>[2x]MEAEKKLFLKALKEKFEEDPKEKYTKFYTFGGWQQSARKREFVEANEKIVAEKRGGIPMYNPDIGVPLGQRKLMPYKLSGTDYIVEGDDLHFMNNAAIQQMWDDIRRTVIVGMDTGHAVLEKRLGVEVTPETINEYMATINHSLPGGAVVQEHMVEVHPSLAWDCYAKIFTGDDELADELDKKYLIDINKLFPEEQAEQLKAAIGKKTYQVSRVPTLVGRVCDGGTIARWSAMQIGMSFITAYKLCAGEAAIADFSYAAKHADVVGVGTALPARRSRGANEPGGIPFGVLCDIVQTTRISDDPVEQSLEVVAVGAMLYDQVWLGSYMSGGVGFTQYATAAYTDDILDDFAYYGYEYVEKKYGINSTKPTMDVVEDIATEVTLYSLEQYDEFPTLLEDHFGGSQRAAVAAAASGISVCMATGNSNAGVNGWYLSQIMHKEYHSRLGFYGYDLQDQCGASNSLSIRNDEASPLELRGPNYPNYAMNVGHQGEYAGITQAAHSARKDAFAMNPLIKIAFADPSLVFDFARPRKECARGALREFEAAGERDVILPAK;>[2x]MVKYEDKISLYDAKGNLVEDGVPLEAISPL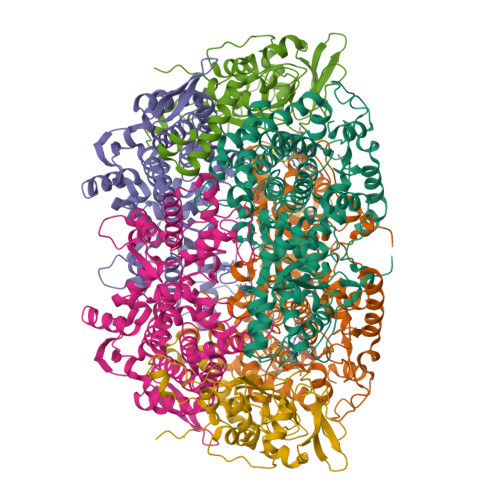YNPTIKAMVKNIKRTVAVNLAGIENSLKTGAIGGKGCKVPGRTLDLPIVENAEAIMDEVEKILRITPDDDTQLRAINDGKQLVVQVPSKRLEVAAEYSVSMLNTAMALKEAIIKTFDVDLFDGSTIHAAIVGRYPQVMDYMGGNIASLLGAPSNMEGLGYALRNIMVNHYVATTKKNLMNAVAFASIMEQTAMFEMGDAIGSFERMHLLGLAYQGLNSDNLVIDLVKANSKGTVGTVVASVVERALEDKVIVEDKSLESGFTMYKPADVAKWNAYAAAGLVAAVIVNCGAARAAQNVASTILYYNDILEYETGLPGTDFGRAEGTAVGFSFFSHSIYGGGGPGIFTGNHVVTRHSKGFAIPPVCAAMCADAGTQMFSPEKTSALVGAVYSAIDEFREPLKYVIEGALEVKDKI;>MAYKPQFYPGATKIAQNRRDHLNPDFELEKLREIPDEELVKVMGHRQPGEDYKTVHPPLEEMDLPEDYVRDLVEPISGAKEGHRIRYIQFADSMYFAPAQPYDRARMYMWRFRGVDTGSLSGRQVIEMRESNLEEISKNVLMDTSLFDPARIGMRGATVHGHSLRLDENGLMFDALQRYVYDEKTGHVVYVKDQVGRPLDEPVDVGEPLPEEKLREITTIYRKDGVPMRDDEELLTVVKRIHRARTLGGYMPVNEVFDKLL[2x]> MFKLKLLSISTIFILAGCVSLAPEYQRPPAPVPQQFSLSKNSLTPAVNSYQDTGWRNFFVDPQVSRLIGEALNN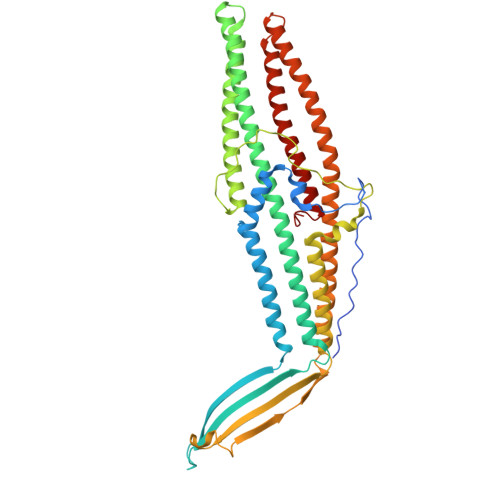NRDLRMAALKVEEARAQFNVTDADRYPQLNASSGITYNGGLKGDKPTTQEYDAGLELSYELDFFGKLKNMSEADRQNYFASEEARRAVHILLVSNVSQSYFSQQLAYEQLRIARETLKNYEQSYAFVEQQLVTGSTNVLALEQARGQIESTRAEIAKREGDLAQANNALQLVLGTYRAVPSEKGIKGGEIAPVKLPPNLSSQILLQRPDIMEAEYQLKAADANIGAARAAFFPSITLTSGLSSSSTELSSLFTSGSGMWNFIPKIEIPIFNAGRNKANLKLAEIRQQQSVVNYEQKIQSAFKDVSDTLALRDSLSQQLESQQRYLDSLQITLQRARGLYASGAVSYIEVLDAERSLFATQQTILDLTYSRQVNEINLFTALGGGWVEK> MADYKDDDDKSGPDEVDASGREEGARHRNNTEKKHPGGGESDASPEAGSGGGGVALKKEIGLVSACGIIVGNIIGSGIFVSPKGVLENAGSVGLALIVWIVTGFITVVGALCYAELGVTIPKSGGDYSYVKDIFGGLAGFLRLWIAVLVIYPTNQAVIALTFSNYVLQPLFPTCFPPESGLRLLAAIC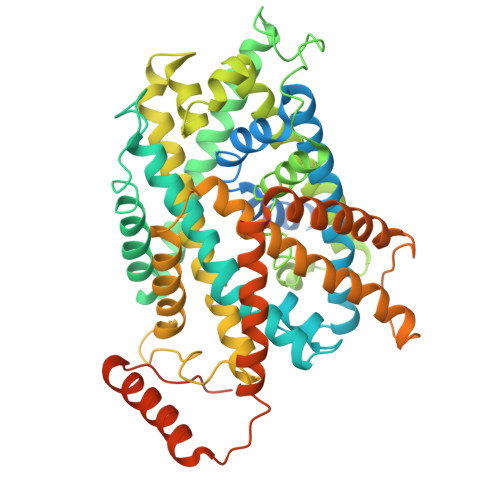LLLLTWVNCSSVRWATRVQDIFTAGKLLALALIIIMGIVQICKGEYFWLEPKNAFENFQEPDIGLVALAFLQGSFAYGGWNFLNYVTEELVDPYKNLPRAIFISIPLVTFVYVFANVAYVTAMSPQELLASNAVAVTFGEKLLGVMAWIMPISVALSTFGGVNGSLFTSSRLFFAGAREGHLPSVLAMIHVKRCTPIPALLFTCISTLLMLVTSDMYTLINYVGFINYLFYGVTVAGQIVLRWKKPDIPRPIKINLLFPIIYLLFWAFLLVFSLWSEPVVCGIGLAIMLTGVPVYFLGVYWQHKPKCFSDFIELLTLVSQKMCVVVYPEVERGSGTEEANEDMEEQQQPMYQPTPTKDKDVAGQPQP The arginine route involves three enzymatic steps: (i) arginine decarboxylation to agmatine by arginine decarboxylase (ADC, EC 4.1.1.19); (ii) deimination of agmatine by agmatine iminohydrolase (AIH, EC 3.5.3.12) and (iii) hydrolysis of N-carbamoylputrescine (NCP) to putrescine by N-carbamoylputrescine amidohydrolase (CPA, EC 3.5.1.53), with the release of carbon dioxide and ammonia. N-carbamoylputrescine amidohydrolase enzymes belong to nitrilases, and more precisely, to C-N hydrolases breaking non-peptide bonds using Cys-Glu-Lys catalytic triad. The octameric MtCPA enzyme is assembled into an incomplete helical twist, made by four tight dimers with swapped C-termini. As in other nitrilases, the substrate hydrolysis is carried out by the catalytic triad, composed in MtCPA of Glu48 (proton acceptor), Lys121 (proton donor) and Cys158 (nucleophile).

Instead, we decided to construct the MtCPA-C158S mutant. Substitution of sulfhydryl with hydroxyl group preserved binding properties of residue 158 but strongly diminished its reactivity. The structure of unliganded MtCPA-C158S, determined at 2.39 Å resolution, presented significantly lower noise in the electron density maps around the active site when compared to the unliganded wild-type MtCPA. This improvement allowed to identify the ligand bound inside the active site as GOL. However, GOL does not penetrate deep inside the pocket and presents no direct interactions with either of the residues from catalytic triad. Instead, it is hydrogen-bonded with the side chain oxygen of Glu187. Considering the fact that in the MtCPA-C158S mutant structure, GOL enters the active site, and mimics the substrate or product, the niche-bound GOL quite likely might represent the secondary binding site.

>SNAMAEDKGRKVVVSALQFACTDDVSTNVTTAERLVRAAHKQGANIVLIQELFEGYYFCQAQREDFIQRAKPYKDHPTIMRLQKLAKELGVVIPVSFFEEANNAHYNSIAIIDADGTDLGIYRKSHIPDGPGYEEKFYFNPGDTGFKVFQTKYAKIGVAISWDQWFPEAARAMALQGAEILFYPTAIGSEPHDQSIDSRDHWKRVMQGHAGANLVPLVASNRIGNEIIETEHGKSEIKFYGNSFIAGPTGEIVSIADDKEEAVLIAEFNLDKIKSMRHCWGVFRDRRPDLYKVLLTLDGKNPVL[16x]>[2x]MAPPNGTTNGETEVATQGSYTAVSTGRKTTMHRLIEEHGSVLMPGVQDALSAAVVEKTGFHAAFVSGYSVSAAMLGLPDFGLLTTTEVVEATRRITAAAPNLCVVVDGDTGGGGPLNVQRFIRELISAGAKGVFLEDQVWPKKCGHMRGKAVVPAEEHALKIAAAREAIGDSDFFLVARTDARAPHGLEEGIRRANLYKEAGADATFVEAPANVDELKEVSAKT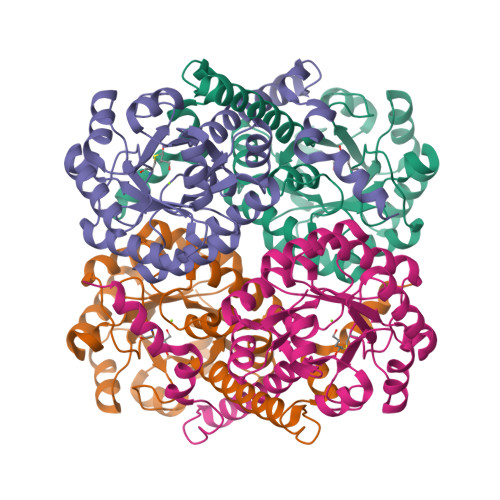KGLRIANMIEGGKTPLHTPEEFKEMGFHLIAHSLTAVYATARALVNIMKILKEKGTTRDDLDQMATFSEFNELISLESWYEMESKFKNFTPKAT5'-O-({1-[(2E)-4-(4-hydroxy-6-methoxy-7-methyl-3-oxo-1,3-dihydro-2-benzofuran-5-yl)-2-methylbut-2-en-1-yl]-1H-1,2,3-triazol-4-yl}methyl)adenosine 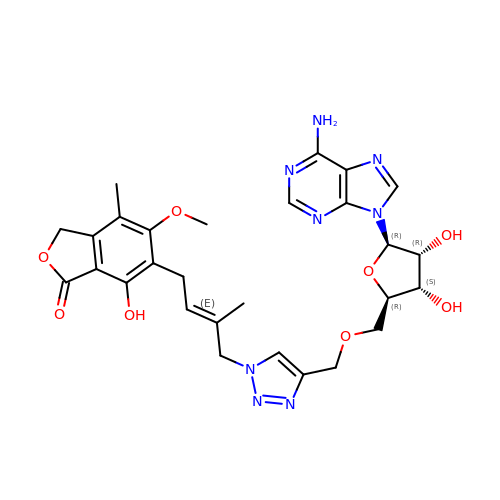| C28 H32 N8 O8 | KHAINKCXZBTBIV-WDLZNNHFSA-N> MAGLAQHIQLKYIFGMNNEIRNSLQFHDEDRIIYPAGYNVVLHDLNDKSQHYYQGTNEYRGISCLALSPLKRYLALGVKGQRDPAIIIFDTFTQKRRKNLGLNLGNLDRYNIKQWVSIAFPSQNQETKYIFSLSGAGGDVVLCWWWHEKGKCLGSIDLGAQNDIYEISFNHSDANSICVTGNNFFGIYAKIEGTYVREDNQQKQKPSVQNGENSSAAQLPQPTLNIQVSAGNNNQNPQPEIKLENGNLISNLPADIVEKNFVAHLWMQCESYLVVFVESGEIILCDSRGNFLQIMEQSPRYFIVSRSGMIKIVAAVAYSKGFYVACSESIVLQYHYTQDNDKNPFTCVNQFKLKQFVELKEIEIKSICMNKAEDKLLIGLDNNQIYEIKIKPYHPETVNNDSSEDREVTLINHLNHTGPINSMDICKRKPIIATCSTDKTIKIWDYEKKQIKISWAFNEEAFCLSLHPQGFCVAVGFLDKLRLMNLCIHNSQNTTKNKAYKEISPFKGCKEIKFSNGGQYFAAVNSTSSNHVIQVFKFFTGENPSQLVFKGHTGRVKCIAWSSDDSFLLSCGLDGMILAWKLDQDFQHQQTIVPRIVDIHNKGVNFSGLTLTVDNKTIVAVGNDRHIHQAVINEQQPVDKTDKKLLDINLSCLAFPSSNKLLFAGIQDDARSSGAIRCFIYPLTHGKFTDYQAHDERGVEKMKITNDDRYIITAGKDGCIMVFEIKDKDARGMKLKDGYAKYSEEELITRSDLDDLKSTRDGLIVQINEFSNQNAMIGLNSRDDRIRQLETQIENNSQKRKQMFEQLLKSKTMEEQKLIQEINEIKEQFEQEIQVMDTKYQ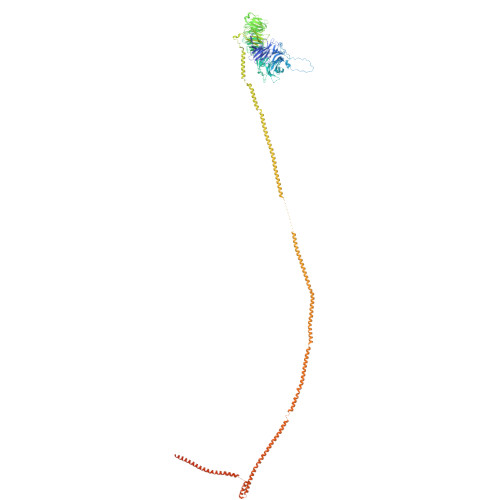KEVMSLVEEYENQKRLHEIENNKNNKKKTKLLQEHSQKLQIIDDQYQKLLEEQITQKERVEKQINHLQKEQQEVLMQISEEKETEIKNLNQKNSKDEQAITDQGLKAKSDISITKKKIMQQQQEAQDLKEQKQEYERQKEKLKIQNQELRDKIDGQKKIILERDRTIGEKEKIIYNLKKKAQDLEKFKFVLDHKIKELKRDIVPREDEITKMKQETNNMDQYLKELNAYNNYLGTVVDELYTTQETMKEDIKQQRQQISVQQVKISRFKDDVYSLAQHILDYDKLVDETERLFMKHVNDKEVKRQSVEGDIMMEYRSQKKNLEKLVNMFKKSLQKDNQIHKDDKIRIMKDNVDLIREINTLRKSIKDITKGQQSNIPDQKGQTQHMPLQTPQLSRKSISQPVLPPISKSAMFEGVTQQNEIQKSHTQINPELVEEKQKVLNSLQTDILELQKVYEALNYEKHNLTQA>[2x]GAMASSSHSRAGQSAAGAAPGGGVDTRDAEMPATEKDLAEDAPWKKIQQNTFTRWCNEHLKCVSKRIANLQTDLSDGLRLIALLEVLSQK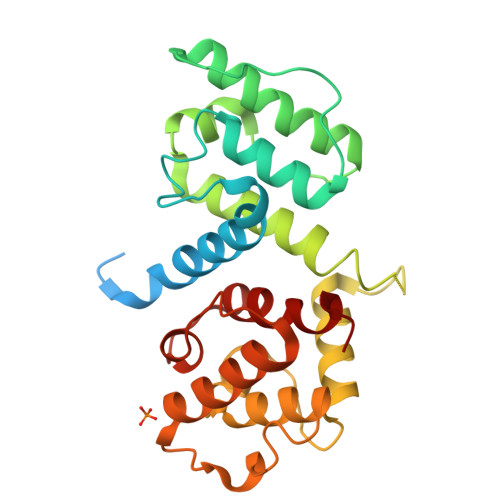KMHRKHNQRPTFRQMQLENVSVALEFLDRESIKLVSIDSKAIVDGNLKLILGLIWTLILHYSISMPMWDEEEDEEAKKQTPKQRLLGWIQNKLPQLPITNFSRDWQSGRALGALVDSCAPGLCPDWDSWDASKPVTNAREAMQQADDWLGIPQVITPEEIVDPNVDEHSVMTYLSQFPKAKL> GGA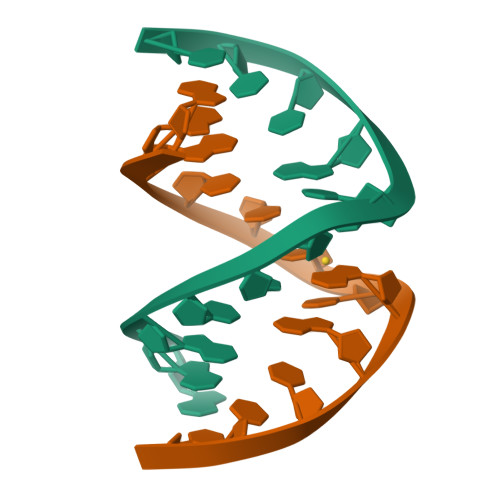CCCCGGTCC>[8x]GPLGSPLTASMLASAPPQEQKQMLGE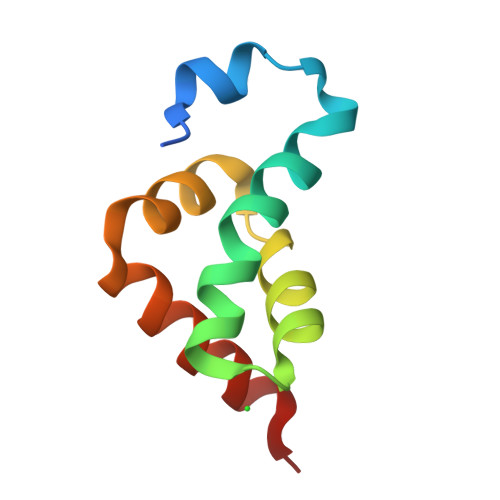RLFPLIQAMHPTLAGKITGMLLEIDNSELLHMLESPESLRSKVDEAVAVLQAH Nucleolar protein 66 (NO66) is a JmjC domain-containing protein which has been reported to be a histone demethylase and a ribosome protein 8 (Rpl8) hydroxylase. Nucleolar protein 66 (NO66) is a metazoan JmjC domain-containing protein that is highly conserved throughout evolution and was initially identified as a dual-location intranuclear protein. Evidence from a recent study indicated that NO66 hydroxylates ribosome protein 8 (Rpl8) and controls the biogenesis of the ribosome, which is consistent with the observation that NO66 is a constitutive nucleolar component. Moreover, previous work demonstrated that NO66 assembles as a tetramer and that the binding site of NO66 to osterix is located on the surface formed by a hinge region (interface I) from neighbouring subunits in the tetramer.

We had already produced two mutant proteins, M1 and M2, lacking dimer interfaces I and II, and they exist as a monomer and a dimer, respectively. To further understand the role of interface II in the regulation of the activity of NO66, we determined the structure of the mutant protein M2 lacking the interface. As predicted, the M2 protein forms a dimer with interface I. The overall structure of monomeric M2 protein is almost identical to wild-type NO66, with an r.m.s.d. of 0.37 Å. Interestingly, when the dimer structure of the M2 protein was superimposed onto the dimer of NO66 coupled in the same way, we found that one of the M2 molecules in the dimer moves outwards compared with the wild-type protein. Interface II, which was deleted in M2, pulls these two subunits towards the other two subunits to form an NO66 tetramer. This tetramerization may further facilitate the shifting of the subunits when NO66 binds to its substrate. In this context, we proposed that oligomerization of NO66 might affect the motion of each subunit in the catalytic process and thus control the activity.

>GGEPAWDSPLRRVLAELNRIPSSRRRAARLFEWLIAPMPPDHFYRRLWEREAVLVRRQDHTYYQGLFSTADLDSMLRNEEVQFGQHLDAARYINGRRETLNPPGRALPAAAWSLYQAGCSLRLLCPQAFSTTVWQFLAVLQEQFGSMAGSNVYLTPPNSQGFAPHYDDIEAFVLQLEGRKLWRVYRPRVPTEELALTSSPNFSQDDLGEPVLQTVLEPGDLLYFPRGFIHQAECQDGVHSLHLTLSTYQRNTWGDFLEAILPLAVQAAMEENVEFRRGLPRDFMDYMGAQHSDSKDPRRTAFMEKVRVLVARLGHFAPVDAVADQRAKDFIHDSLPPVLTDRERALSVYGGGGQLTTETEVHMLQDGIARLVGEGGHLFLYYTVENSRVYHLEEPKCLEIYPQQADAMELLLGSYPEFVRVGDLPCDSVEDQLSLATTLYDKGLLLTKMPLALN[2x]> IFEERHLKYISQLGKGNFGSVELCRYDPLGDNTGALVAVKQLQHSGPDQQRDFQREIQILKALHSDFIVKYRGVSYGPGEPSLRLVMEYLPSGCLRDFLQRHRARLDASRLLLYSSQICKGMEYLGSRRCVHRDLAARNILVESEAHVKIADFGLAKLLPLDKDYYVVREPGQSPIFWYAPESLSDNIFSRQSDVWSFGVVLYELFTYCDKSCSPSAEFL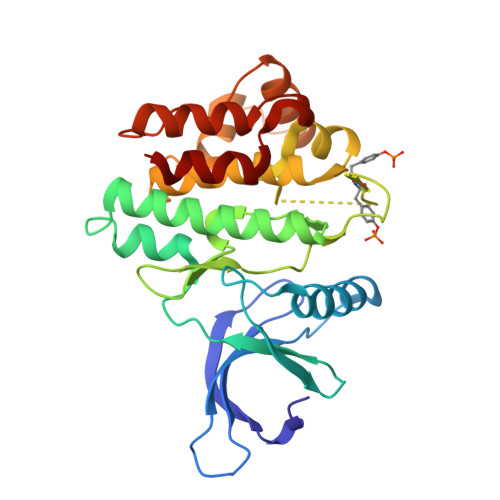RMMGSERDVPALSRLLELLEEGQRLPAPPACPAEVHELMKLCWAPSPQDRPSFSALGPQLDML>KKIFKPEELRQALMPTLEALYRQDPESLPFRQPVDPQLLGIPDYFDIVKNPMDLSTIKRKLDTGQYQEPWQYVDDVWLMFNNAWLYNRKTSRVYKFCSKLAEVFEQEIDPVMQSLG[2x]

Many proteins, including the EP300/CBP histone acetyltransferases (HATs), contain several targetable domains. EP300 and CBP broadly regulate the activity of other proteins through their protein acetyltransferase catalytic activity. These proteins contain several highly homologous domains, including KIX, bromodomains (BRDs) and HAT domains, through which they interact with, dock to, and acetylate target proteins, respectively. EP300/CBP are critical gene-regulatory targets in cancer, with existing high potency inhibitors of either the catalytic HAT domain or protein-binding bromodomain (BRD). Using crystallography, we identify the binding mechanism of the EP300/CBP-specific BRD inhibitor CCS1477 in complex with the EP300, CBP and BRD4 BRDs, and define components of the CCS1477 catalytic binding core that are required for compound activity.

The resultant compounds displayed a >1000-fold loss of affinity for EP300 and CBP. A co-crystal structure of the CBP bromodomain with compound 1 demonstrated that the side chain R1173 is more flexible than in co-crystal structures with CCS1477 and assumes a conformation incompatible for hydrogen-bonding with the piperidinone oxygen, while weakly interacting with a nitrogen of the benzimidazole core. Therefore, loss of Pi-cation as well as hydrogen-bonding interactions renders compounds 1 and 2 less efficient binders to EP300 and CBP. Notably, activity against BRD4 was reduced by ~10-fold, indicating that the hydrophobic van-der-Waals (VDW) interactions observed between the difluorophenyl moiety of CCS1477 and the WPF shelf of BRD4 contribute to binding affinity, but relatively less so in the EP300/CBP bromodomain. To further evaluate the specific effects of CCS1477-int(1) as a case example, we performed further CellTiter-Glo dose-response growth assays in HDMB03 and MB002 G3MB cells, demonstrating a blunting of anti-growth effect in cells treated with CCS1477-int(1), as compared with CCS1477. Thus, the difluorophenyl group is a critical moiety in the CCS1477 pharmacophore that facilitates potent interaction with the bromodomain of EP300/CBP and is required for efficacy in cell line models of G3MB.> KTSDANETEDHLESLICKVGEKSACSLESNLEGLAGVLEADLPNYKSKILRLLCTVARLLPEKLTIYTTLVGLLNARNYNFGGEFVEAMIRQLKESLKANNYNEAVYLVRFLSDLVNCHVIAAPSMVAMFENFVSVTQEEDVPQVRRDWYVYAFLSSLPWVGKELYEKKDAEMDRIFANTESYLKRRQKTHVPMLQVWTADKPHPQEEYLDCLWAQIQKLKKDRWQERHILRPYLAFDSILCEALQHNLPPFTPPPHTEDSVYPMPRVIFRMFDYTDDPEGPVMPGSHSVERFVIEENLHCIIKSHWKERKTCAAQLVSYPGKNKIPLNYHIVEVIFAELFQLPAPPHIDVMYTTLLIELCKLQP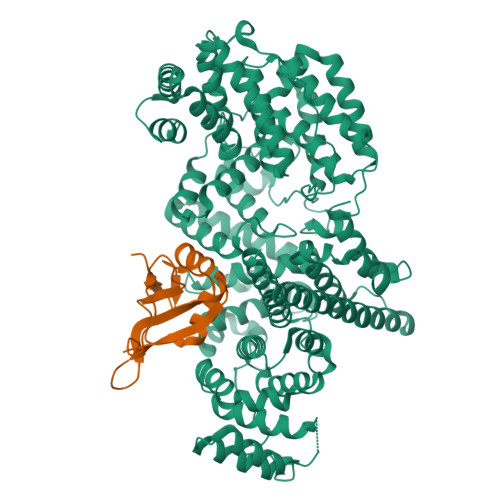GSLPQVLAQATEMLYMRLDTMNTTCVDRFINWFSHHLSNFQFRWSWEDWSDCLSQDPESPKPKFVREVLEKCMRLSYHQRILDIVPPTFSALCPSNPTCIYKYGDESSNSLPGHSVALCLAVAFKSKATNDEIFSILKDVPNPNQDDDDDEGFSFNPLKIEVFVQTLLHLAAKSFSHSFSALAKFHEVFKTLAESDEGKLHVLRVMFEVWRNHPQMIAVLVDKMIRTQIVDCAAVANWIFSSELSRDFTRLFVWEILHSTIRKMNKHVLKIQKELEEAKEKLARQHKRRSDDDDRSSDRKDGVLEEQIERLQEKVESAQSEQKNLFLVIFQRFIMILTEHLVRCETDGTSVLTPWYKNCIERLQQIFLQHHQIIQQYMVTLENLLFTAELDPHILAVFQQFCALQA;> MSGGLLKALRSDSYVELSQYRDQHFRGDNEEQEKLLKKSCTLYVGNLSFYTTEEQIYELFSKSGDIKKIIMGLDKMKKTACGFCFVEYYSRADAENAMRYINGTRLDDRIIRTDWDAGFKEGRQYGRGRSGGQVRDEYRQDYDAGRGGYGKLAQNQ Pinoresinol/lariciresinol reductase (PLR), an NADPH-dependent reductase, converts pinoresinol to lariciresinol and subsequently to secoisolariciresinol. Here, we present crystal structures of IiPLR1 from Isatis indigotica and pinoresinol reductases (PrRs) AtPrR1 and AtPrR2 from Arabidopsis thaliana, in the apo, substrate-bound and product-bound states. The crystal structures were captured in the apo, substrate-bound and/or product-bound forms. We found that, for all 16 structures we solved, each enzyme adopts a similar head-to-tail dimer conformation, strongly suggesting that each PLR/PrR functions as a homodimer, consistent with the literature that TpPLR1 exists as a dimeric entity in solution. Each structure contains a head-to-tail homodimer, and the catalytic pocket comprises structural elements from both monomers. β4 loop covers the top of the pocket, and residue 98 from the loop governs catalytic specificity.

Intriguingly, the β4 loop is well defined in the AtPrR1_NAP structure but disordered in the AtPrR1/2_apo structures. These structural differences suggest that the loops are somewhat flexible, and act as a switch to control the binding of NADPH and release of NADP+.

>[4x]MGESKRTEKTRVLVVGATGYIGKRIVRACLAEGHETYVLQRPEIGLEIEKVQLFLSFKKLGARIVEGSFSDHQSLVSAVKLVDVVVSAMSGVHFRSHNILVQLKLVEAIKEAGNVKRFLPSEFGMDPPRMGHALPPGRETFDQKMEVRQAIEAAGIPYTYVVGACFAAYFAGNLSQMVTLLPPKEKVNIYGDGNVKVVFADEDDIAKYTAKTLNDPRTLNKTVNIRPPDNVLTQLELVQIWEKLTGKELEKTNIAAQDFLANIEQMEIPHQAGIGHFYHIFYEGCLTDHEVGEDEEASSLYPDVKYKRMDDYLRMFL>[2x]MGSSHHHHHHSSGLVPRGSHMPSYTVTVATGSQEHAGTDDYIYLSLVGSAGCSEKHLLDKGSFERGAVDSYDVTVDEELGEIQLVRIEKRKYGSNDDWYLKYITLKTPHGDYIEFPCYRWITGDVEVVLRDGRAKLARDDQIHILKQHRRKELETRQKQYRWMEWNPGFPLSIDAKCHKDLPRDIQFDSEKGVDFVLNYSKAMENLFINRFMHMFQSSWNDFADFEKIFVKISNTISERVMNHWQEDLMFGYQFLNGANPVLIRRCTELPEKLPVTTEMVECSLERQLSLEQ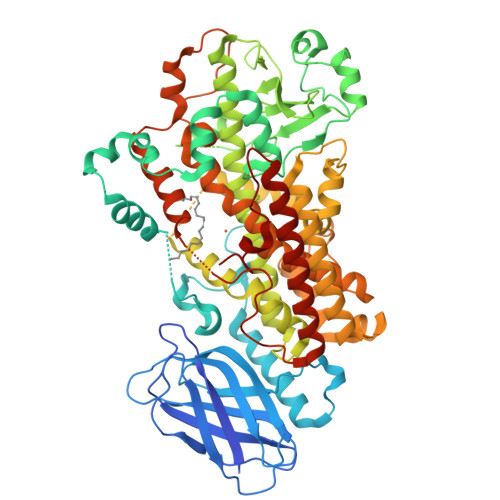EVQQGNIFIVDFELLDGIDANKTDPCTLQFLAAPICLLYKNLANKIVPIAIQLNQIPGDENPIFLPSDAKYDWLLAKIWVRSSDFHVHQTITHLLRTHLVSEVFGIAMYRQLPAVHPIFKLLVAHVRFTIAINTKAREQLICECGLFDKANATGGGGHVQMVQRAMKDLTYASLCFPEAIKARGMESKEDIPYYFYRDDGLLVWEAIRTFTAEVVDIYYEGDQVVEEDPELQDFVNDVYVYGMRGRKSSGFPKSVKSREQLSEYLTVVIFTASAQHAAVNFGQYDWASWIPNAPPTMRAPPPTAKGVVTIEQIVDTLPDRGRSCWHLGAVWALSQFQENELFLGMYPEEHFIEKPVKEAMARFRKNLEAIVSVIAERNENLQLPYYYLDPDRIPNSVAI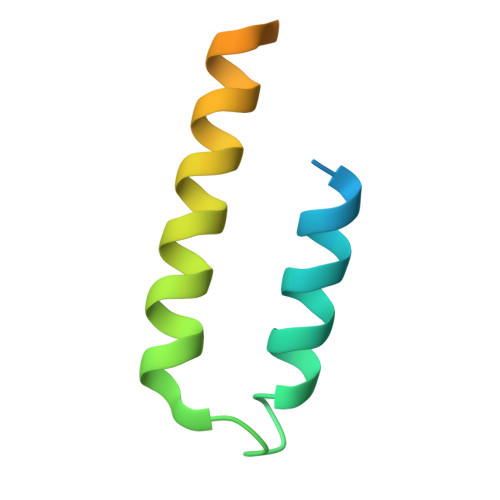> MLFFKEKFYNELSYYRGGHKDLESMFELALEYIEKLEEEDEQQVTDYENAMEEELRDAVDVIESQLEIIKDIVR>MADLLANIDLKKADGTVKKGSDALANKKVVALY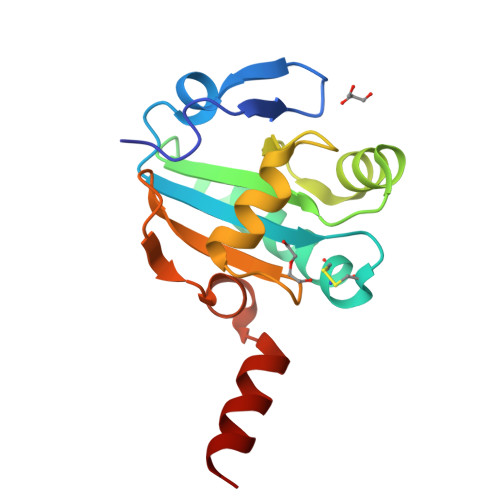FSAHWCPPCRQFTPILKEFYEEVDDDQFEIVFVSLDHSEEDLNNYVKESHGDWYHVPFGSSEIEKLKNKYEVAGIPMLIVIKSDGNVITKNGRADVSGKAPPQTLSSWLAAA[3x]> AQDDSTPDSLFAGLVGEYYGTNSQLNNISDFRALVDSKEADATFEAANISYGRGSSDVAKGTHLQEFLGSDASTLSTDPGDNTDGGIYLQGYVYLEAGTYNFKVTADDGYEITINGNPVATVDNNQSVYT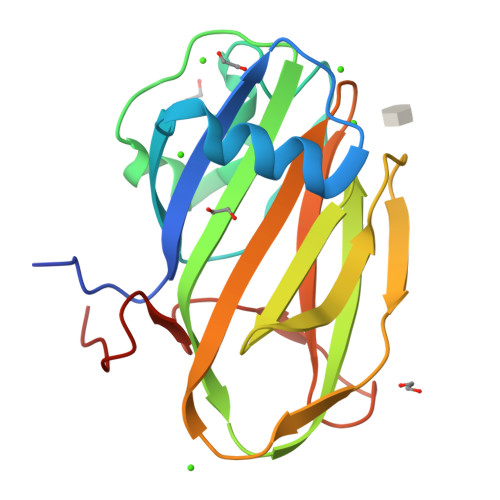VTHASFTISESGYQAIDMIWWDQGGDYVFQPTLSADGGSTYFVLDSAILSSTGETPYTTAQ>[6x]MSLIDPRAIIDPSARLAADVQVGPWSIVGAEVEIGEGTVIGPHVVLKGPTKIGKHNRIYQFSSVGEDTPDLKYKGEPTRLVIGDHNVIREGVTIHRGTVQDRAETTIGDHNLIMAYAHIGHDSVIGNHCILVNNTALAGHVHVDDWAILSGYTLVHQYCRIGAHSFSGMGSAIGKDVPAYVTVFGNPAEARSMNFEGMRRRGFSSEAIHALRRAYKVVYRQGHTVEEALAELAESAAQFPEVAVFRDSIQSATRGITR

LpxA and LpxD are functionally and structurally similar, sharing a homotrimer architecture and conserved active site features, especially in the acyl-chain binding pockets that reside in the dimer interface of the β-helix trimer core. Herein we report the discovery of several small molecules that bind to both P. aeruginosa LpxA and LpxD with μM affinity, identified using a targeted structure-based methodology that utilizes molecular docking, surface plasmon resonance (SPR) bioanalysis, and high-resolution X-ray crystallography.

For compound 1, the complex structure with LpxA was solved at 2.10 Å resolution. Two modes of binding conformations can be identified in terms of the relative location of the carboxyl group, with minor variations in the positioning of the carboxyl group seen within each bind mode. In the first binding mode (exemplified by pose 1), the carboxyl group is within hydrogen bonding distance to the Gln157 main chain and His156 side chain. In the other binding mode (exemplified by pose 2), the ligand’s carboxyl group is positioned near the Gln157 side chain, forming a hydrogen bond. The rest of compound 1, including the carbonyl group and the naphthalene ring, is placed identically in all poses. Notable intermolecular interactions include a hydrogen bond between the carbonyl oxygen and the Gly151 main chain. Additionally, the naphthalene ring forms multiple non-polar interactions with residues His118, Asn133, Val132, Ala136, Ala138, and Met169. Among these, Met169 is the so-called “hydrocarbon ruler” that ensures the length of the incoming acyl chain substrate is no longer than 10 carbon atoms. Aside from the acyl-chain binding pocket, compound 1 was found in a second binding pocket outside the active site at the dimer interface, where a second copy of the substrate UDP-GlcNAc was also identified in the previously published LpxA-substrate complex structure. The naphthalene ring of compound 1 forms non-polar interactions with Leu3, Gly23 and Pro24, whereas the carboxyl group establishes favorable electrostatic interactions with Arg57.>IRVFAIPPSFASIFLTKSTKLTCLVTDLTTYDSVTISWTRQNGEAVKTHTNISESHPNATFSAVGEASICEDDWNSGERFTCTVTHTDLPSPLKQTISRPKGVALHRPDVYLLPPAREQLNLRESATITCLVTGFSPADVFVQWMQRGQPLSPEKYVTSAPMPEPQAPGRYFAHSILTVSEEEWNTGETYTCVVAHEALPNRVTERTVDKSTGKPTLYNVSLVMSDTAGTCY[10x];> EDERIVLVDNKCKCARITSRIIRSSEDPNEDIVERNIRIIVPLNNRENISDPTSPLRTRFVYHLSDLCKKCDPTEVELDNQIVTATQSNICDEDSATETCYTYDRNKCYTAVVPLVYGGETKMVETALTPDACYPD;> RILPEVKVEGELGGSVTIKCPLPEMHVRIYLC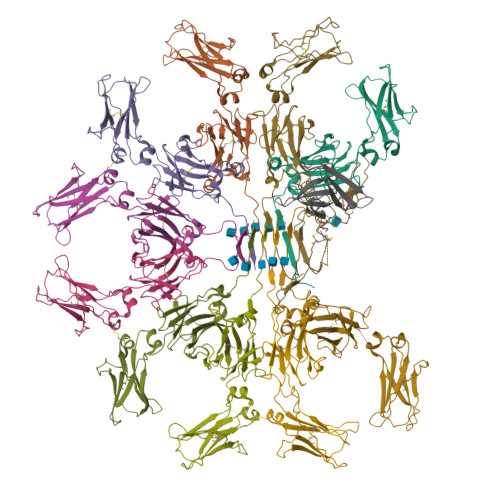REMAGSGTCGTVVSTTNFIKAEYKGRVTLKQYPRKNLFLVEVTQLTESDSGVYACGAGMNTDRGKTQKVTLNVHS2-(benzyloxy)benzohydrazide | C14 H14 N2 O2 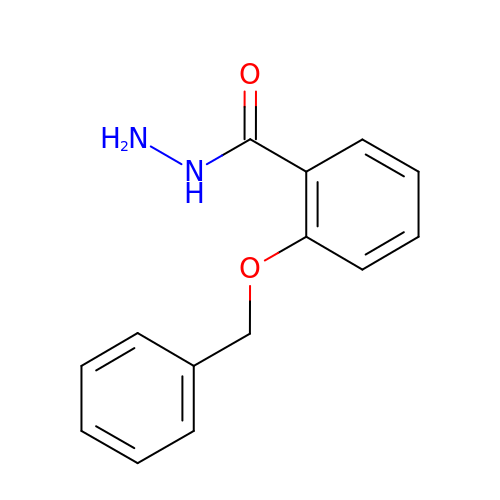| WPIKJQNXQSBHPU-UHFFFAOYSA-N> MHHHHHHDYKDDDDKENLYFQGRDPTQFEERHLKFLQQLGKGNFGSVEMCRYDPLQDNTGEVVAVKKLQHSTEEHLRDFEREIEILKSLQHDNIVKYKGVCYSAGRRNLK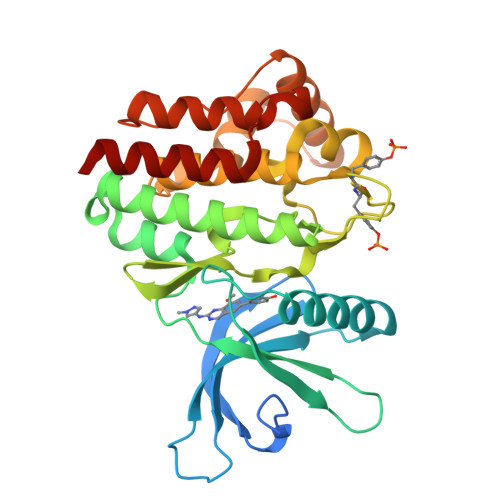LIMEYLPYGSLRDYLQKHKERIDHIKLLQYTSQICKGMEYLGTKRYIHRDLATRNILVENENRVKIGDFGLTKVLPQDKEYYKVKEPGESPIFWYAPESLTESKFSVASDVWSFGVVLYELFTYIEKSKSPPAEFMRMIGNDKQGQSIVTHLIELLKNNGRLPRPDGCPDEIYMIMTECWNNNVNQRPSFRDLALRVDQIRDNMAG>[2x]TTNKPIVLSTWNFGLHANVEAWKVLSKGGKALDAVEKGVRLVEDDPTERSVGYGGRPDRDGRVTLDACIMDENYNIGSVACMEHIKNPISVARAVMEKTPHVMLVGDGALEFALSQGFKKENL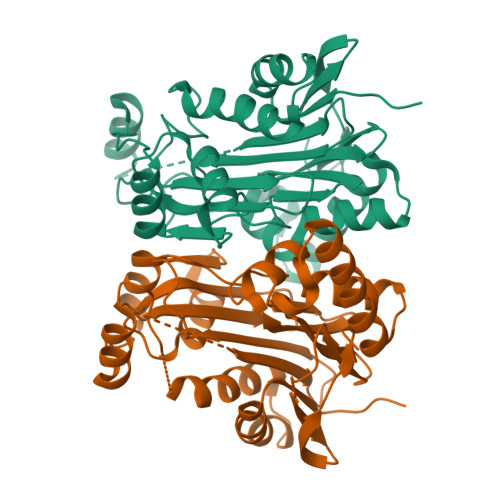LTAESEKEWKEWLKTSQYKPIVNIENHDTIGMIALDAQGNLSGACTTSDMAYKMHGRVGDSPIIGAGLFVDNEIGAATATGHGEEVIRTVGTHLVVELMNQGRTPQQACKEAVERIVKIVNRRGKNLKDIQVGFIALNKKGEYGAYCIQDGFNFAVHDQKGNRLETPGFALK>SK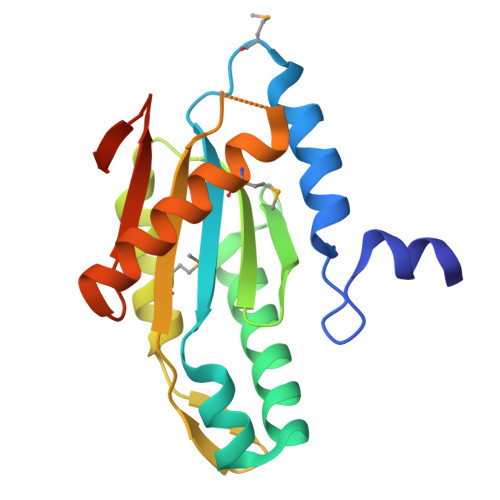LEFLAFYDELTGLPNKNSLIRWLNLKVSQMDCIDTYLIFLEVRDLEKLNVTYGYDLVDELIIHISKRIKDIAGEGNKAFKIGFDRFAIICKSENISDFIERMLSQLLLPYNVNGNLIRVNFNIGAAQIENSNEAAANLMRRCDLALIKAKEEGLNEYVIFKPSIEIQTLEHHHHHH[2x]>MSINSREVLAEKVKNAVNNQPVTDMHTHLFSPNFGEILLWDIDELLTYHYLVAEVMRWTDVSIEAFWAMSKREQADLIWEELFIKRSPVSEACRGVLTCLQGLGLDPATRDLQVYREYFAKKTSEEQVDTVLQLANVSDVVMTNDPFDDNERISWLEGKQPDSRFHAALRLDPLLNEYEQTKHRLRDWGYKVNDEWNEGSIQEVKRFLTDWIERMDPVYMAVSLPPTFSFPEESNRGRIIRDCLLPVAEKHNIPFAMMIGVKKRVHPALGDAGDFVGKASMDGVEHLLREYPNNKFLVTMLSRENQHELVVLARKFSNLMIFGCWWFMNNPEIINEMTRMRMEMLGTSFIPQHS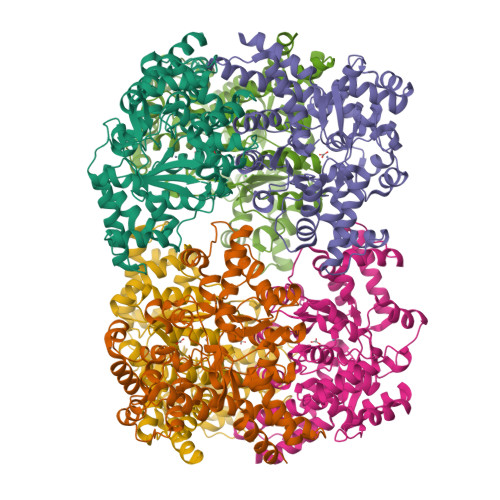DARVLEQLIYKWHHSKSIIAEVLIDKYDDILQAGWEVTEEEIKRDVADLFSRNFWRFVGRNDHVTSVKVEQQT[2x]Here, we show that thermophilic viruses have appropriated the SAVED domain of CalpL as an anti-CRISPR, AcrIII-2 (second anti-CRISPR of type III systems), which they use to degrade cA4. AcrIII-2 dimers sandwich cA4, degrading it in a shared active site to short linear products, using a mechanism highly reminiscent of CalpL. Here, we demonstrate that the viral protein binds and degrades cyclic tetra-adenylate (cA4), generating linear products, similar to the ring nuclease activity of the CalpL protein.

The structure of AcrIII-2, solved by molecular replacement with X-ray crystallography with data to 1.79 Å resolution, revealed two molecules in the asymmetric unit. Each molecule resembles a canonical SAVED subunit, which sits in a head-to-tail configuration. The structure of an AcrIII-2 monomer comprises two CARF-like domains tethered by a 19-residue loop. Each CARF domain contains a five-stranded β-sheet sandwiched between three α-helices; strands 1 to 4 of the β-sheet lie parallel, whilst the fifth strand is anti-parallel. The loop fusing the domains is followed by a six-residue β-strand that lies anti-parallel to the first β-strand of the canonical C-terminal CARF domain, in essence making this a six-stranded β-sheet. The crystal structure of AcrIII-2 revealed a dimeric composition in the absence of cA4, with SAVED subunits orientated similarly to that observed in the cryoEM structure of the CalpL filament bound to cA4. Coupled with the observation of a dimeric species formed by cross-linking in the absence of cA4, these data suggest that apo AcrIII-2 dimerises, and it is likely the dimers and longer filaments are stabilised upon cA4 binding. It does, however, demonstrate that the global orientation of the two AcrIII-2 SAVED domains is not significantly different from the SAVED domains of CcaCalpL, meaning AcrIII-2 was highly likely to bind cA4 at the dimer interface.

>GANAMAHMIGVYITKWGFEVETFKKALPKNTEVKTIAFTGDWIEAVRQFYSTVKEIDGHIHLALNGPSSLAFGCGVIFGSLKTFSFWHYQNGAYHTIPITNVRALKQRLKQYNYVEPFYEAGGKDLVVMLNYSHHEIKTAVKEYVMNKLRLENPSYLEISLKGITGNIPIELMPTVANETSSLLQDVKKHQSFDRFHFFFSCPVPIAFMVGVAFGLYDELVVYNFSGTYEPVLSFKDLKEVKL[2x]> SQSNRELVVDFLSYKLSQKGYSWSQFSDVEENRTEAPEETEAERETPSAINGNPSWHLADSPAVNGATGHSSSLDAREVIPMAAVKQALREAGDEFELRYRRAFSDLTSQLHITPGTAYQSFEQVVNELFRDGVNWGRIVAF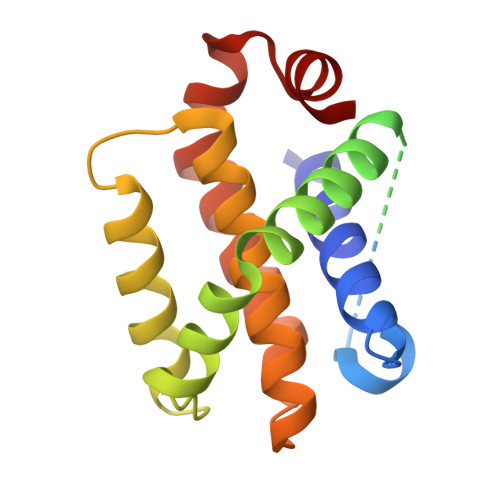FSFGGALCVESVDKEMQVLVSRIASWMATYLNDHLEPWIQENGGWDTFVDLYG>[2x]SNAMVKMLVLYYSAYGYMEQMAKAAAEGAREGGAEVTLKRVPELVPEEVAKASHYKIDQ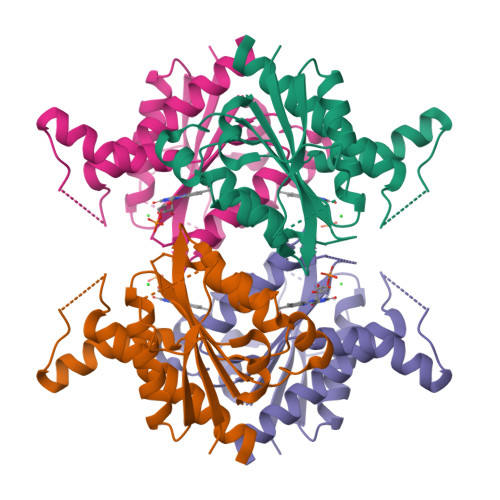EVPIATPGELADYDAIIIGTATRYGMMASQMKNFLDQTGGLWAKGALINKVGSVMVSTATQHGGAELALISTQWQMQHHGMIIVPLSYAYREQMGNDVVRGGAPYGMTTTADGDGSRQPSAQELDGARFQGRRVAEITAKLHG> MNTNNIKKYAPQARNDFRDAVIQKLTTLGIAADKKGNLQIAEAETIGETVRYGQFDYPLSTLPRRERLVKRAREQGFEVLVEHCAYTWFNRLCAIRYMELHGYLDHGFRMLSHPETPTAFEVLDHVPEVAEALLPESKAQLVEMKLSGNQDEALYRELLLGQCHALHHAMPFLFEAVDDEAELLLPDNLTRTDSILRGLVDDIPEEDWEQVEVIGWLYQFYISEKKDAVIGKVVKSEDIPAATQLFTPNWIVQYLVQNSVGRQWLQTYPDSPLKDKMEYYIEPAEQTPEVQAQLAAITPASIEPESIKVLDPACGSGHILTEAYNVLKAIYEERGYRTRDIPQLILENNIFGLDIDDRAAQLSGFAMLMLARQDDRRILGRGVRLNIVSLQESKLDIAEVWTKLNF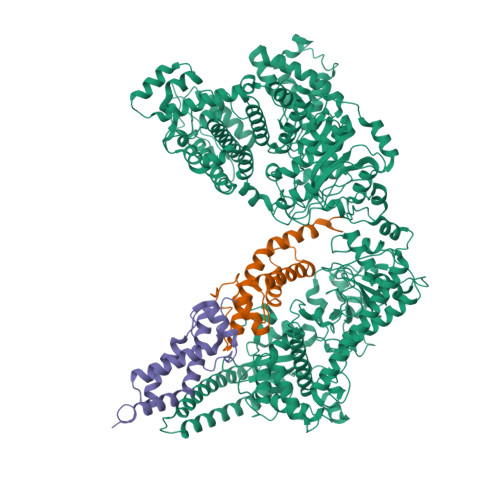HQHMQRGSMGDMFTQGTALANTDSAEYKLLMRTLALFTSAKTLGSLIQVPQEDEAALKAFLEGLYRLAVEGDIQQKEAAAELIPYIQQAWILAQRYDAVVANPPYMGGKGMNGDLKEFAKKQFPDSKSDLFAMFMQHAFSLLKENGFNAQVNMQSWMFLSSYEALRGWLLDNKTFITMAHLGARAFGQISGEVVQTTAWVIKNNHSGFYKPVFFRLVDDNEEHKKNNLLNRMNCFKNTLQNDFKKIPGSPIAYWATLAFINSFLKLPALGTRAVKGLDTNGSIDVFLRRWPEVSINSFDALGKGNSKWFPIAKGGELRKWFGNHEYIINYENDGIELRKNKANLRNKDMYFQEGGTWTVVSTTGFSMRYMPKGFLFDQGGSAVFCENNDELSIYNILACMNSKYINYSASLICPTLNFTTGDVRKFPVIKNNHLEDLAKKAIEISKADWNQFETSWEFSKNKLIEHKGNVAYSYASYCNFQDKLYEQLVNIEKNINNIIEEILGFKIETTENSELITLNSNKIYRYGQSETNDTFLNRHRSDTISELISYSVGCQMGRYSLDREGLVYAHEGNKGFADLVAEGAYKTFPADSDGILPLMDDEWFEDDVTSRVKEFVRTVWGEEHLQENLEFIAESLCLYAIKPKKGESALETIRRYLSTQFWKDHMKMYKKRPIYWLFSSGKEKAFECLVYLHRYNDATLSRMRTEYVVPLLARYQANIDRLNDQLDEASGGEATRLKRERDSLIKKFSELRSYDDRLRHYADMRISIDLDDGVKVNYGKFGDLLADVKAITGNAPEVI;>[2x]MAMSNMTYNNVFDHAYEMLKENIRYDDIRDTDDLHDAIHMAADNAVPHYYADIFSVMASEGIDLEFEDSGLMPDTKDVIRILQARIYEQLTIDLWEDAEDLLNEYLEEVEEYEEDEE~{N}-[5-(4-oxidanylidene-3-propyl-quinazolin-6-yl)pyridin-2-yl]pentanamide | C21 H24 N4 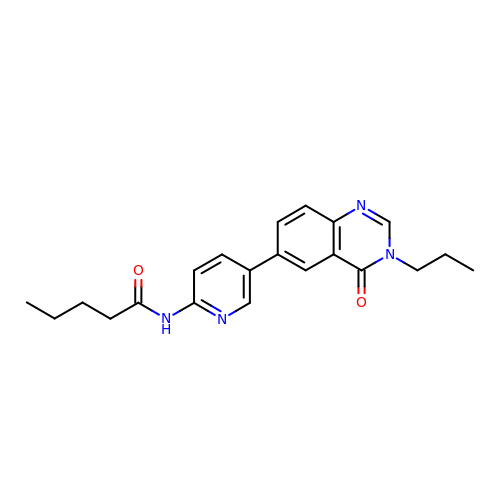O2 | CMSIAWXDJIGAGC-UHFFFAOYSA-N> GGGGUUAUGUGUGCCCGGCAUGGGUGCAGUCUAUAGGGUGAGAGUCCCGAACUGUGAAGGCAGAAGUAACAGUUAGCCUAACGCAAGGGUGUCCGUGGCGACAUGGAAUCUGAAGGAAGCGGACGGCAAACCUUCGGUCUGAGGAACACGAACUUCAUAUGAGGCUAGGUAUCAAUGGAUGAGUUUGCAUAACAAAACAAAGUCCUUUCUGCCAAAGUUGGUACAGAGUAAAUGAAGCAGAUUGAUGAAGGGAAAGACUGCAUUCUUACCCGGGGAGGUCUGGAAACAGAAGUCAGUAGAAGUCAUAGUACCCUGUUCGCAGGGGAAGGACGGAACAAGUAUGGCGUUCGCGCCUAAGCUUGAACUGCCGUAUACCGAACGGUACGUACGGUAGUGUG

Group II introns are ubiquitous self-splicing ribozymes and retrotransposable elements evolutionarily and chemically related to the eukaryotic spliceosome, with potential applications as gene-editing tools. The site also harbors a metal-ion cluster formed by two divalent (M1–M2) and two monovalent (K1–K2) ions. In the first step of splicing, depending on whether the intron follows a hydrolytic or a transesterification mechanism, respectively, a water molecule or the 2′-OH group of a bulged adenosine in D6, activated by M2 and by the triple helix, attack the 5′-splice junction of the precursor (5e-I-3e), forming an intron/3′-exon intermediate (I-3e), in which the scissile phosphate (SP) is coordinated by K2. In the second step of splicing, the 5′-exon (5e), activated by M1, performs a nucleophilic attack on the 3′-splice junction, releasing ligated exons (5e-3e) and a linear or lariat form of the excised intron.

After incorporating the resulting triple base mutations (C289A/C358A/G385U, aka the A-mutant; C289G/C358G/G385C, aka the G-mutant; and C289U/C358U/G385A, aka the U-mutant), we monitored effects on splicing kinetics. We then determined the crystal structures of the G and U mutants in the presence of sodium and magnesium at 3.2 and 3.3 Å resolution, respectively. However, the detailed architecture of the active site differs significantly from wild type under sodium conditions. By contrast with wild type, the G and U mutants in sodium maintain the triple helix configuration, as revealed by the Fo − Fc maps calculated by omitting the J2/3 residues and the catalytic metals (total peak height for the triple helix conformer of the G288 nucleobase = 7.5 σ in the G-mutant and = 9.3 σ in the U-mutant). Therefore, these structures show that the G and U mutants are unable to adopt the toggled conformation, which may explain their tendency to stall after the first step of splicing. We found that the A-mutant—which can be protonated at position 358—splices at rates comparable to wild type, whereas the G and U mutants—which cannot be protonated at position 358—have splicing defects. Most remarkably, both G and U mutants show accumulation of linear I-3e intermediate, which indicates that these mutants stall after the first step of splicing and have difficulty progressing into the second step. We noted that the K1–N7G288 interaction was not stably formed in the mutants, preventing K1 release. Finally, the crystallographic data suggest that the G and U mutants do not sample the toggled conformation, thus impairing a critical rearrangement of the intron active site between the two steps of splicing.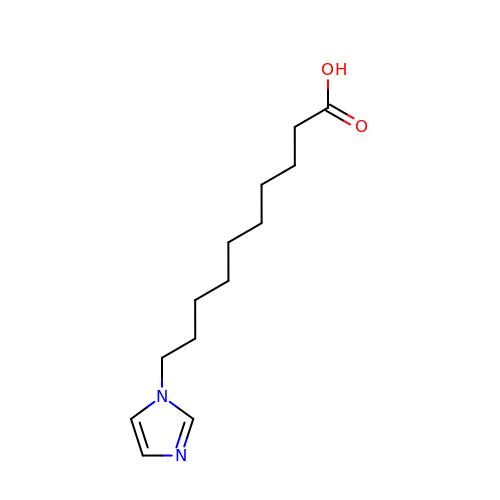10-(1H-imidazol-1-yl)decanoic acid | C13 H22 N2 O2 | DOJPUPKORVKCJK-UHFFFAOYSA-N>GSSGKNDESGIPIANAKLDDVADLLGGALFLPLYKWMNEYGPIYRLAAGPRNFVIVSDPAIAKHVLRNYPKYAKGLVAEVSEFLFGSGFAIAEGPLWTARRRAVVPSLHRRYLSVIVERVFCKCAERLVEKLQPYAEDGSAVNMEAKFSQMTLDVIGLSLFNYNFDSLTTDSPVIEAVYTALKEAELRSTDLLPYWKIDALCKIVPRQVKAEKAVTLIRETVEDLIAKCKEIVEREGERINDEEYVNDADPSILRFLLASREEVSSVQLRDDLLSMLVAGHETTGSVLTWTLYLLSKNSSALRKAQEEVDRVLEGRNPAFEDIKELKYITRCINESMRLYPHPPVLIRRAQVPDILPGNYKVNTGQDIMISVYNIHRSSEVWEKAEEFLPERFDIDGAIPNETNTDFKFIPFSGGPRKCVGDQFALMEAIVALAVFLQRLNVELVPDQ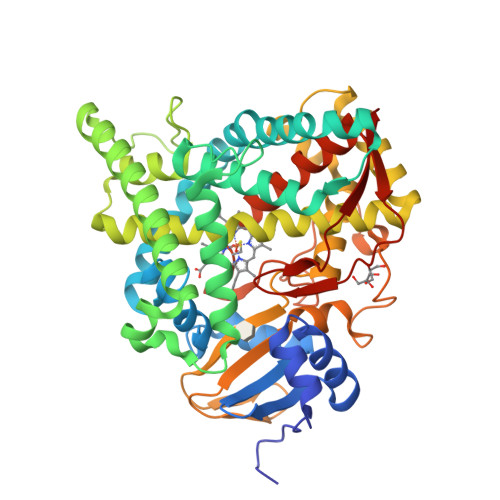TISMTTGATIHTTNGLYMKVSQR[4x]>[4x]RRLETQKEAEANRGYGKPSLGGPFHLEDMYGNEFTEKNL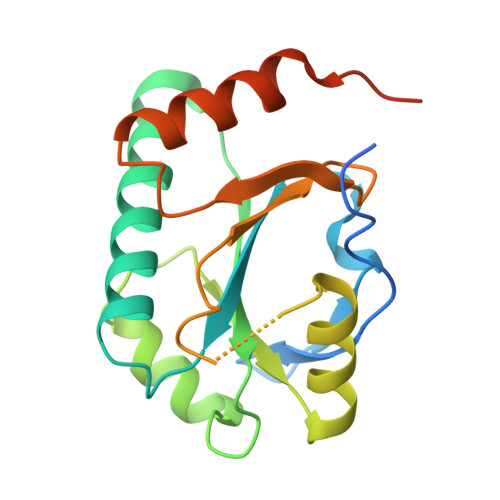LGKFSIIYFGFSNCPDICPDELDKLGLWLNTLSSKYGITLQPLFITCDPARDSPAVLKEYLSDFHPSILGLTGTFDEVKNACKKYRVYFSTPPNVKPGQDYLVDHSIFFYLMDPEGQFVDALGRNYDEKTGVDKIVEHVKSYVPAEQRAKQKEAWYSFLFK>[3x]GPQKRCLFVCRHGERMDVVFGKYWLSQCFDAKGRYIRTNLNMPHSLPQRSGGFRDYEKDAPITVFGCMQARLVGEALLESNTVIDHVYCSPSLRCVQTAHNILKGLQQDNHLKIRVEPGLFEWTKWVAGSTLPAWIPPSELAAANLSVDTTYRPHIPVSKLAISESYDTYINRSFQVTKEIISECKSKGNNILIVAHASSLEACTCQLQGLSPQNSKDFVQMVRKIPYLGFCSCEELGETGIWQLTD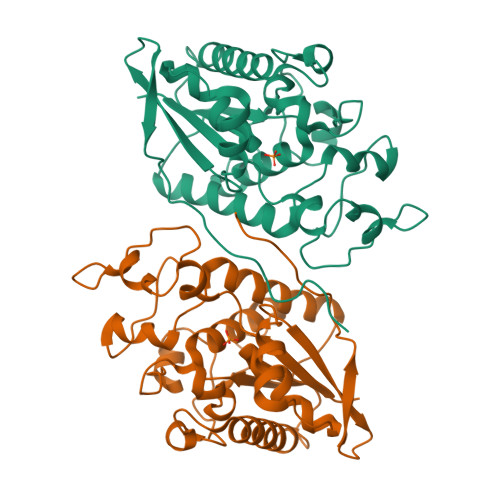PPILPLTHGPTGGFNWRETLLQE> WQPPWYCKEPVRIGSCKKQFSSFYFKWTAKKCLPFLF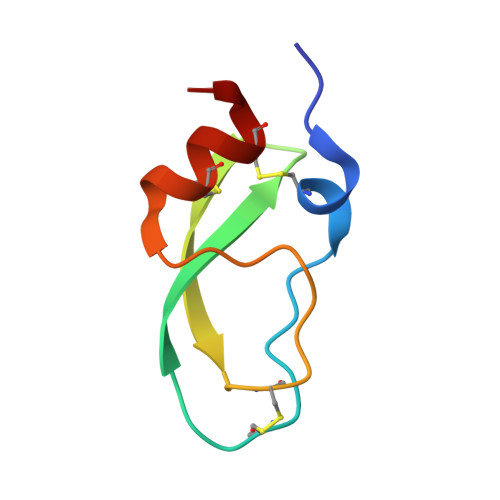SGCGGNANRFQTIGECRKKCLGK Lmb, a laminin binding adhesin of S. agalactiae is a surface associated 34 kDa lipoprotein. It mediates streptococcal adherence to laminin isolated from host placental membranes and is also important for the invasion of human brain endothelial cells. Lmb is made of two domains with (α/β)4 topology and the domains are connected by a long disordered loop. Close to this loop, at the interface of the two domains, a zinc binding site is observed where the Zn2+ ion is coordinated by three histidines (His66, His142 and His206) and a glutamate (Glu281).

In order to elucidate the role of the flexible loop (Gly123-Leu138) in metal binding and laminin binding, a construct (ΔLmb) was made, replacing the loop region with a short linker (PGATV) and its structure was determined by molecular replacement using wt Lmb as a model. On comparison with wt Lmb, the backbone structure of ΔLmb including the regions at either ends of the deleted loop remains unaffected. These two structures superpose with an rms deviation of 0.4 Å for 247 Cα atoms. Surprisingly, the ΔLmb structure showed the presence of bound zinc, in contrast to two other deletion mutant structures of SBPs, namely ZnuA-Se and ZnuA-Syn, which were devoid of metal ion at the active site. However, only the primary zinc binding site has been located and no such secondary site is observed in Lmb, possibly because of the absence of histidines in the loop, which cannot coordinate an additional zinc ion. Another notable feature in ΔLmb is the packing of the two monomers in the crystallographic asymmetric unit which is different from that of the wt Lmb. In ΔLmb, the truncated loops of the two molecules face each other and form the interface. In contrast, in wt Lmb, the two monomers are oriented such that the loops face away from each other. A similar difference in the packing of the monomers in the crystal lattice was observed between wt and ΔZnuA-Syn. It is noteworthy to mention that both wt and ΔLmb exist as a dimer in solution, as shown by gel filtration experiments, although the physiological relevance of such a dimeric assembly is not known. Our data conclusively shows that the loop spanning residues Gly123-Leu138 do not play a significant role in metal acquisition and the interaction with laminin.

>[2x]GMSVVTSFYPMYAMTKEVSGDLNDVRMIQSGAGIHSFEPSVNDVAAIYDADLFVYHSHTLEAWARDLDPNLKKSKVNVFEASKPLTLDRVKPGATVYDPHTWTDPVLAGEEAVNIAKELGHLDPKHKDSYTKKAKAFKKEAEQLTEEYTQKFKKVRSKTFVTQHTAFSYLAKRFGLKQLGISGISPEQEPSPRQLKEIQDFVKEYNVKTIFAEDNVNPKIAHAIAKSTGAKVKTLSPLEAAPSGNKTYLENLRANLEVLYQQLK>[24x]MTSAEMTSPNNNSEHQAIAKMRTMIEGFDDISHGGLPIGRSTLVSGTSGTGKTLFSIQFLYNGIIEFDEPGVFVTFEETPQDIIKNARSFGWDLAKLVDEGKLFILDASPDPEGQEVVGGFDLSALIERINYAIQKYRARRVSIDSVTSVFQQYDASSVVRRELFRLVARLKQIGATTVMTTERIEEYGPIARYGVEEFVSDNVVILRNVLEGERRRRTLEILKLRGTSHMKGEYPFTITDHGINIFPLGAMRLTQRSSNVRVSSGVVRLDEMCGGGFFKDSIILATGATGTGKTLLVSRFVENACANKERAILFAYEESRAQLLRNAYSWGMDFEEMERQNLLKIVCAYPESAGLEDHLQIIKSEINDFKPARIAIDSLSALARGVSNNAFRQFVIGVTGYAKQEEITGLFTNTSDQFMGAHSITDSHISTITDTIILLQYVEIRGE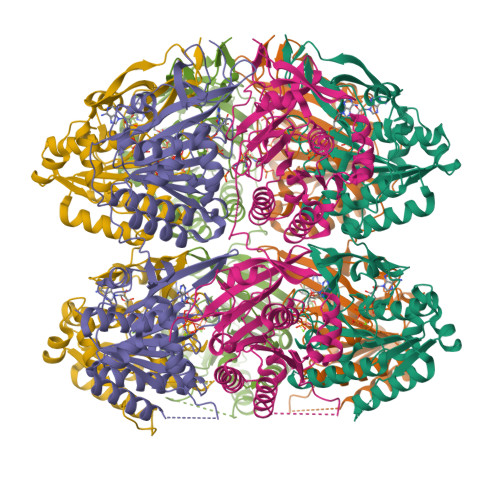MSRAINVFKMRGSWHDKAIREFMISDKGPDIKDSFRNFERIISGSPTRITVDEKSELSRIVRGVQEKGPES N~2~-phosphono-L-leucinamide | C6 H15 N2 O4 P | 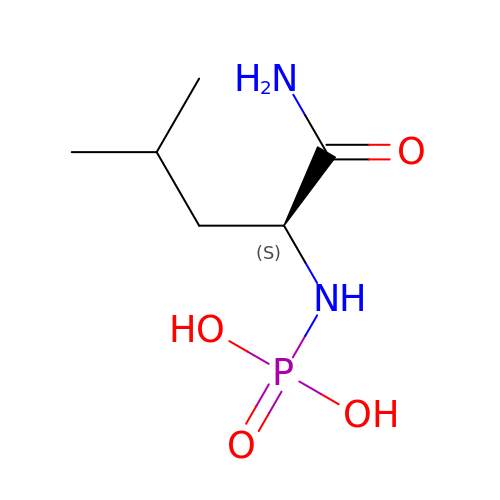LHNDGZQCKJAVRF-YFKPBYRVSA-N>MSFSSKPTVLASRVESDSAINVMKWKTVSTIFLVVVLYLIIGATVFKALEQPQEISQRTTIVIQREKFLRAHPCVSDQELDELIQQIVAADNAGIIPLGASSNQVSHWDLGSSFFFAGTVITTIGFGNISPRTEGGKIFCIIYALLGI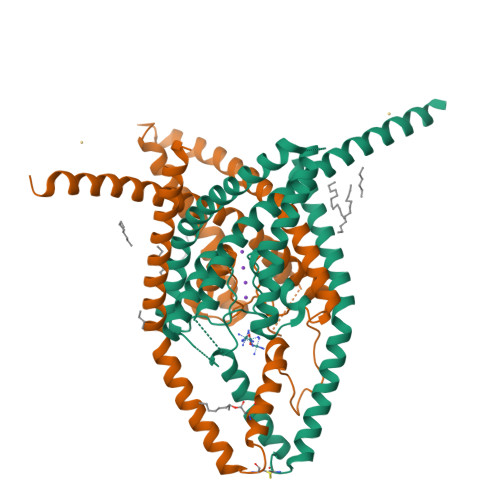PLFGFLLAGVGDQLGTIFGKGIAKVEDTFIKWNVSQTKIRIISTIIFILFGCVLFVALPAVIFKHIEGWSALDAIYFVVITLTTIGFGDYVAGGSDIEYLDFYKPVVWFWILVGLAYFAAVLSMIGDWLRVIAKKTKEAVGEFRAHAAEWTANVTSNSLEVLFQ[2x]>MPQSKSRKIAILGYRSVGKSSLTIQFVEGQFVDSYDPTIENTFTKLITVNGQEYHLQLVKTAGQDEYSIFPQTYSIDINGYILVYSVTSIKSFEVIKVIHGKLLDMVGKVQIPIMLVGNKKDLHMERVISYEEGKALAESWNAAFLESSAKENQTAVDVFRRIILEAEKLEHHHHHH[2x]

Mammalian target of rapamycin complex 1 (mTORC1) serves as a central regulator of cell growth and proliferation by integrating signals from growth factors, nutrients, energy status, and cellular stress. A small GTPase, called Ras homolog enriched in brain (Rheb), is a positive regulator of mTORC1. Like other small GTPases, the function of Rheb is dictated by its guanine nucleotide binding states: it is active in the GTP-bound form and inactive in the GDP-bound form. The Y35N mutant assumes a very similar overall structure as the WT Rheb with a typical small GTPase protein fold composed of a six-stranded β-sheet surrounded by four α-helices.

On the other hand, the D60K mutant was shown to be unable to bind to Mg2+ or the nucleotide (either GTP or GDP) and hence to assume a nucleotide-free form; thus, it is regarded as a dominantly inactive mutant and widely used as a negative control in the functional study of mTORC1 activation (Tabancay et al., 2003). In contrast, the dominantly inactive D60K mutant cannot activate mTORC1 in the presence of either GppNHp or GDP. To investigate the molecular basis for the incapability of the D60K mutant to activate mTORC1, we determined the crystal structure of D60KGDP at 2.6 Å resolution. Surprisingly, there is a GDP bound at the active site of the D60K mutant with clearly defined electron density, even though no GDP was added in the protein purification and crystallization processes, which is in disagreement with the previous functional data showing that the D60K mutant assumes a nucleotide-free form. Nevertheless, consistent with the previous functional data, there is no Mg2+ bound at the active site (Tabancay et al., 2003). Intriguingly, attempts to co-crystallize the D60K mutant with GppNHp failed to yield any crystals. In the D60KGDP structure, the long, positively charged side chain of Lys60 is extended into the Mg2+-binding site, which not only hinders the Mg2+ binding owing to electrostatic repulsion but also expels the side chain of Thr38 away from the active site, to adopt a conformation similar to that seen in WTGDP but different from that seen in Y35NGDP. In addition, distinct from all known WT and mutant Rheb structures, in the D60KGDP structure, a portion of switch I (residues 35 and 36) is disordered.> MEQRTEEWFAARLGKVTASRVADVMTKTKSGYAASRQNYMAELI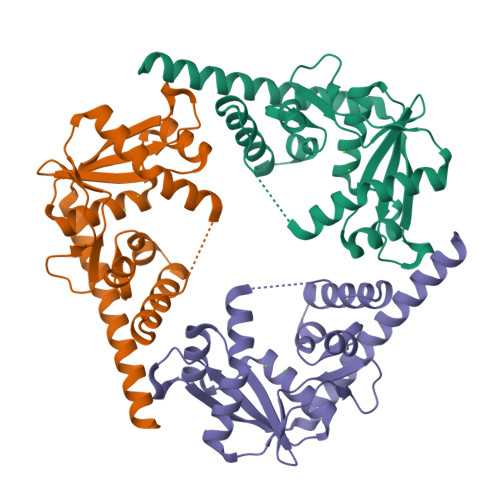CQRLTGTQEIRFSNAAMQRGTELEPHARARYIIETGEIVTEVGLIDHPTIAGFGASPDGLVGDTGLIEIKCPNTWTHIETIKTGKPKPEYIKQMQTQMACTGRQWCDFVSYDDRLPDDMQYFCTRIERDDALIAEIETEVSAFLAELEAEIEYLKRKAAKLAAALEHHHHHH> IVGGTASVRGEWPWQVTLHTTSPTQRHLCGGSIIGNQWILTAAHCFYGVESPKILRVYSGILNQAEIKEDTSFFGVQEII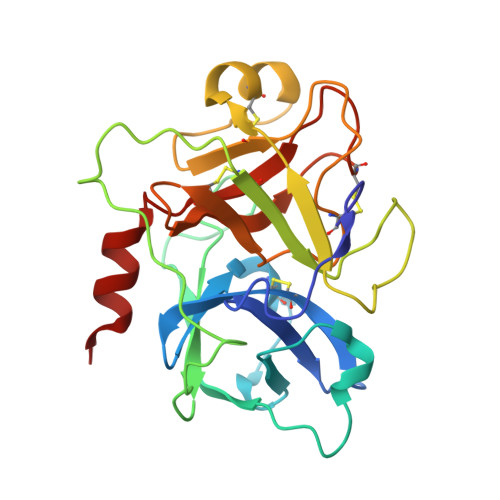IHDQYKMAESGYDIALLKLETTVNYADSQRPISLPSKGDRNVIYTDCWVTGWGYRKLRDKIQNTLQKAKIPLVTNEECQKRYRGHKITHKMICAGYREGGKDACKGDSGGPLSCKHNEVWHLVGITSWGEGCAQRERPGVYTNVVEYVDWILEKTQA>MGSSHHHHHHSSGRENLYFQGMATFVKDLLDRKGRDVVTVGPDVSIGEAAGTLHAHKIGAVVVTDADGVVLGIFTERDLVKAVAGQGAASLQQSVSVAMTKNVVRCQHNSTTD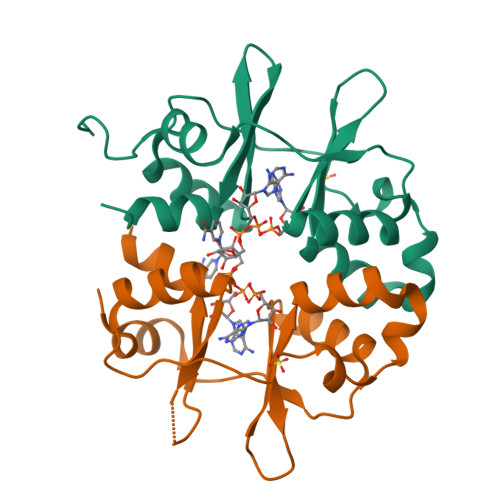QLMEIMTGGRFRHVPVEENGRLAGIISIGDVVKARIGEIEAEAEHIKAYIAG[4x]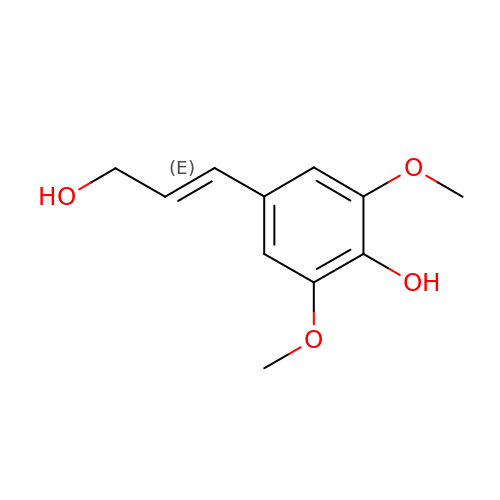4-[(1E)-3-hydroxyprop-1-en-1-yl]-2,6-dimethoxyphenol | C11 H14 O4 | LZFOPEXOUVTGJS-ONEGZZNKSA-N>[5x]GSHMDGTEKWRFKTGKAIEASPVIGEDGTIYVGSNDGHLYAINPDGTEKWRFKTGKAI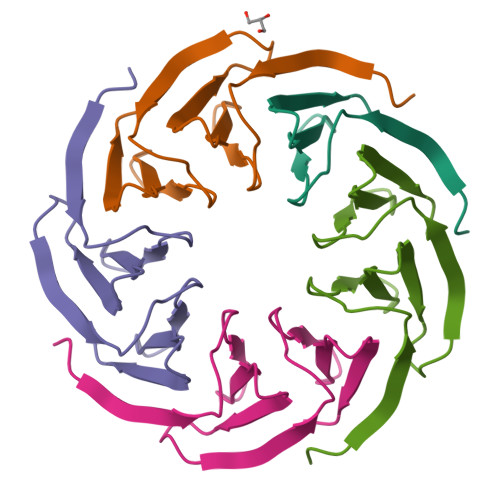EASPVIGEDGTIYVGSNDGHLYAINP>GSHMCLVCSDEASGCHYGVLTCGSCKVFFKRAVEGRQHNYLCAGRNDCIIDKIRRKNCPACRYRKCLQAGMNLEARKTKKKIKGIQQATA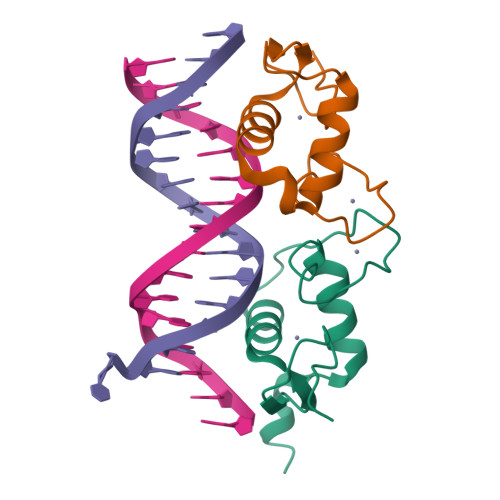G[2x]>MAEHEQVNWPYVNTKLKRDPAVEAQIEKLLAKMTIEQKVAQMIQPEIGYLTVEQMRKYGFGSYLNGGNTAPYGNKRADQATWLKYADEMYLAAMDSTLDGIAIPTVWGTDAMHGHSNVYGATLFPHNIGLGAARDTDLIKRIGQATAKEVAATGIEWSFAPTVAVVRDDRWGRTYESYSEDPDLVKRYAGEMVTGIQGDVGADFLKGSNRIATAKHFVGDGGTERGVDRGNTLIDEKGLRDIHSAGYFSAINQGVQSVMASFNSWNGKRVHGDKHLLTDVLKNQLGFDGFVVSDWNAHKFVEGCDLEQCAQAINAGVDVIMVPEHFEAFYHNTVKQVKAGVIAESRINDAVRRFLRAKIRWGVFTKSKPSARPESQHPQWLGAAEHRTLAREAVRKSLVLLKNNESILPIKASSRILVAGKGANAINMQAGGWSVSWQGTDNTNSDFPNATSIFSGLQSQVTKAGGKITLSESGEYTSKPDVAIVVIGEEPYAEWFGDIELLEFQHETKHALALLKQLKADNIPVVTVFL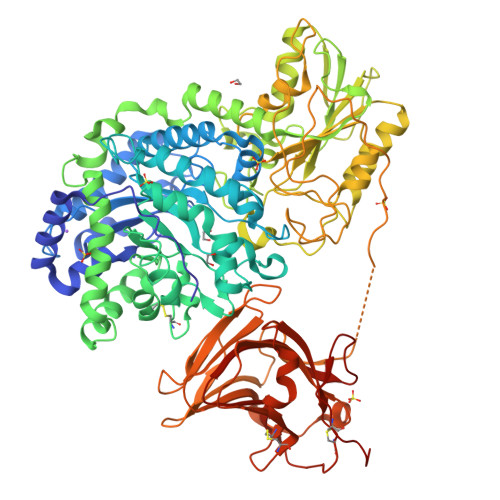SGRPLWVNKELNASDAFVAAWLPGSEGEGVADVLLTNKQGKTQFDFTGKLSFSWPKYDDQFTLNLNDADYDPLFAYGYGLTYQDNINVPVLSEKTSPKKTVNSDSHPLFVRSLAKNMTWQLADTSTQKVLASGASATSGDKQSLLMQSVNLSYQEDGRGFNWRAQAALSLSYLEPTPLDSKFSTGYLELKMRIDKAPEQGANLQVMCSESNCLRDIDFSSFSQLMADKSWHTLAIPLHCDDSDQAEQPITDALRITSQNLSLAIADVALTIKPSDDSISLTCAKLEHHHHHH[4x]>[4x]SNAASMNQLIQAQKKLLPDLLLVMQKRFEILQYIRLTEPIGRRSLSASLGI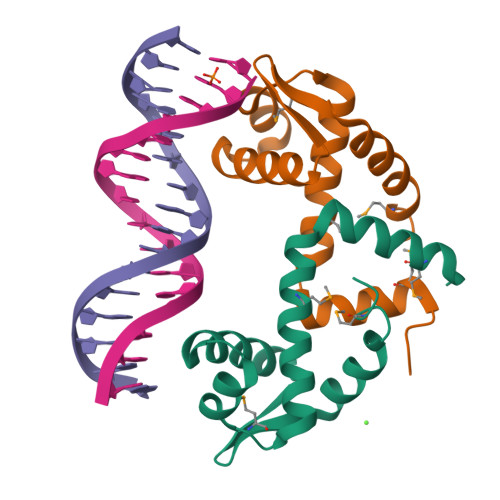SERVLRGEVQFLKEQNLVDIKTNGMTLTEEGYELLSVLEDTMKDV>ATQGVFTLPANTRFGVTAFANSS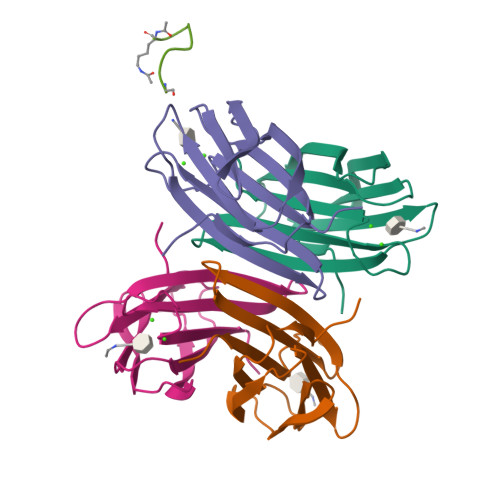GTQTVNVLVNNETAATFSGQSTNNAVIGTQVLNSGSSGKVQVQVSVNGRPSDLVSAQVILTNELNFALVGSEDGTDNDYNDAVVVINWPLG[4x];> KPACYACKA;>KKKK[3x]>GHLPKPTLWAEPGSVIIQGSPVTLRCQGSLQAEEYHLYRENKSASWVRRIQEPGKNGQFPIPSITWEHAGRYHCQYYSHNHSSEYSDPLELVVTGAYSKPTLSALPSPVVTLGGNVTLQCVSQVAFDGFILCKEGEDEHPQCLNSHSHARGWSWAIFSVGPVSPSRRWSYRCYAYDSNSPYVWSLPSDLLE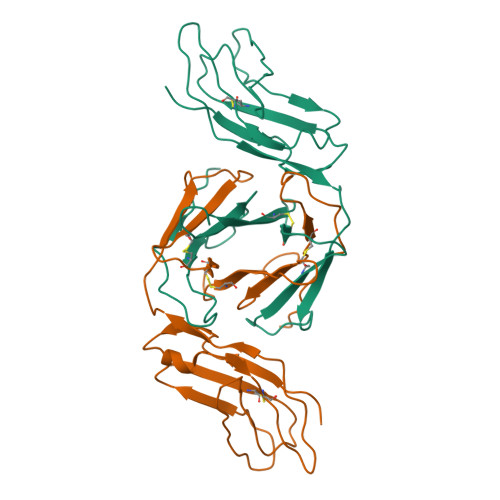LLVPG[2x]> GAPGIAGRIVVLDPGHNGANDSSINNQVPDGRGGTKSCQTSGTATDGGYPEHTFTWNTVLLIRQQLTQLGVRTAMTRGDDNKLGPCIDKRAEIENSYNPDAVVSIHADGGPAGGHGFHVNYSNPPVNAVQGEPTLRFAKTMR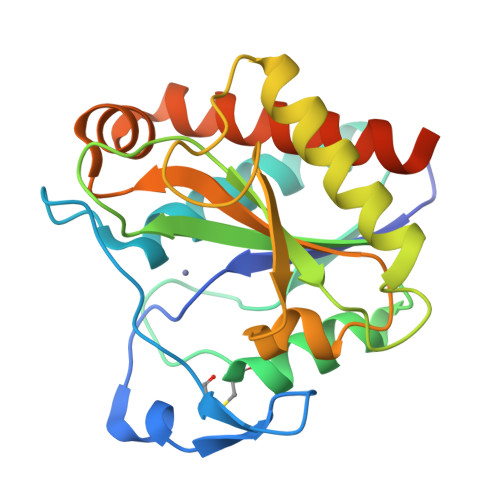DSLQAAGLTPATYIGTGGLYGRSDLAGLNLAQHPKVLVELGNMKNAQDSAMMTSPEGRSKYAQAVVQGIVAYLSGTAPAAAPAPEAAPAGG> DAVQKMLGHCTFEPAEPKAAKNTYTA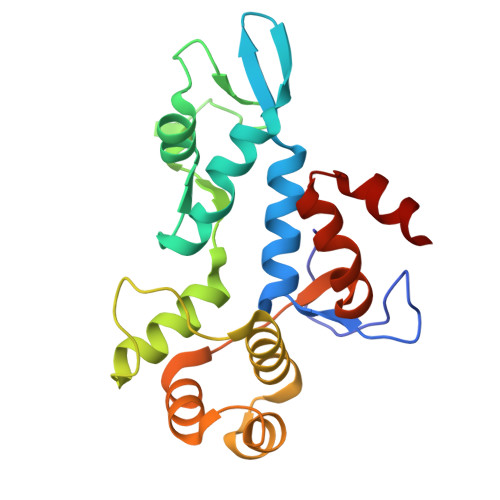ERFIWLTKLNNLRILEQGSERPLTDTERATLMDEPYRKSKLTYAQARKLLGLEDTAFFKGLRYGKDNAEASTLMEMKAYHAISRALEKEGLKDKKSPLNLSPELQDEIGTAFSLFKTDEDITGRLKDRIQPEILEALLKHISFDKFVQISLKALRRIVPLMEQGKRYDEACAEIY> MNIPQRQFSNEEVNRCYLRWQHLRNEHGMNAPSVPEFIYLTKVLQFAAKQRQELQMQRQQQGISGSQQNIVPNSSDQAELPNNASSHISASASPHLAPNMQLNGNETFSTSAHQSPIMQTQMPLNSNGGNNMLPQRQSSVGSLNATNFSPTPANNGENAAEKPDNSNHNNLNLNNSELQPQNRSLQEHNIQDSNVMPGSQINSPMPQQAQMQQAQFQAQQAQQAQQAQQAQQAQARLQQGRRLPMTMFTAEQSELLKAQITSLKCLVNRKPIPFEFQAVIQKSINHPPDFKRMLLSLSEFARRRQPTDQNNQSNLNGGNNTQQPGTNSHYNNTNTDNVSGLTRNAPLDSKDENFASVSPAGPSSVHNAKNGTLDKNSQTVSGTPITQTESKKEENETISNVAKTAPNSNKTHTEQNNPPKPQKPVPLNVLQDQYKEGIKVVDIDDPDMMVDSFTMPNISHSNIDYQTLLANSDHAKFTIEPGVLPVGIDTHTATDIYQTLIALNLDTTVNDCLDKLLNDECTESTRENALYDYYALQLLPLQKAVRGHVLQFEWHQNSLLTNTHPNFLSKIRNINVQDALLTNQLYKNHELLKLERKKTEAVARLKSMNKSAINQYNRRQDKKNKRLKFGHRLIATHTNLERDEQKRAEKKAKERLQALKANDEEAYIKLLDQTKDTRITHLLRQTNAFLDSLTRAVKDQQKYTKEMIDSHIKEASEEVDDLSMVPKMKDEEYDDDDDNSNVDYYNVAHRIKEDIKKQPSILVGGTLKDYQIKGLQWMVSLFNNHLNGILADEMGLGKTIQTISLLTYLYEMKNIRGPYLVIVPLSTLSNWSSEFAKWAPTLRTISFKGSPNERKAKQAKIRAGEFDVVLTTFEYIIKERALLSKVKWVHMIIDEGHRMKNAQSKLSLTLNTHYHADYRLILTGTPLQNNLPELWALLNFVLPKIFNSVKSFDEWFNTPFANTGGQDKIELSEEETLLVIRRLHKVLRPFLLRRLKKDVEKELPDKVEKVVKCKMSALQQIMYQQMLKYRRLFIGDQNNKKMVGLRGFNNQIMQLKKICNHPFVFEEVEDQINPTRETNDDIWRVAGKFELLDRILPKLKATGHRVLIFFQMTQIMDIMEDFLRYINIKYLRLDGHTKSDERSELLRLFNAPDSEYLCFILSTRAGGLGLNLQTADTVIIFDTDWNPHQDLQAQDRAHRIGQKNEVRILRLITTNSVEEVI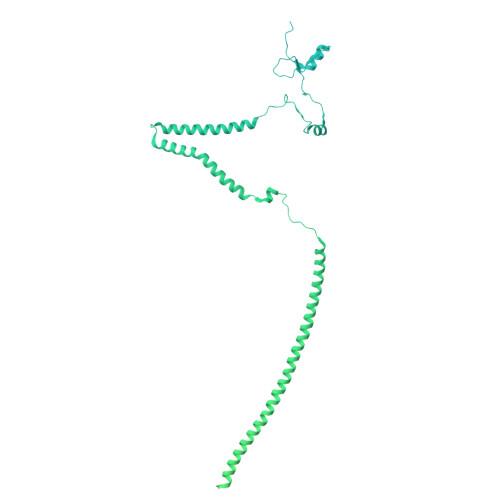LERAYKKLDIDGKVIQAGKFDNKSTSEEQEALLRSLLDAEEERRKKRESGVEEEEELKDSEINEILARNDEEMAVLTRMDEDRSKKEEELGVKSRLLEKSELPDIYSRDIGAELKREESESAAVYNGRGARERKTATYNDNMSEEQWLRQFEVSDDEKNDKQARKQRTKKEDKSEAIDGNGEIKGENIDADNDGPRINNISAEDRADTDLAMNDDDFLSKKRKAGRPRGRPKKVKLEGSENSEPPALESSPVTGDNSPSEDFMDIPKPRTAGKTSVKSARTSTRGRGRGRGRGRGRGRGRGRPPKARNGLDYVRTPAAATSPIDIREKVAKQALDLYHFALNYENEAGRKLSDIFLSKPSKALYPDYYMIIKYPVAFDNINTHIETLAYNSLKETLQDFHLIFSNARIYNTEGSVVYEDSLELEKVVTKKYCEIMGDNSQLDFTEFDEQYGTRPLVLPPVVTSSVAESFTDEADSSMTEASV>SNAMTNQDRPMKSMSESKCYKNRQVFPQDTNHHHTMFGGTLMANIDEIAAITAMKHAGAQVVAASTDSVDFLKPIKTGDILQYVAMVSYAGTSSMEVVVQIRIDDVFNNKHDLAALSYLTFVALDDEGKPKHVPGVYPEDDVEKWFYDTAPQRVERRKARRIESKQ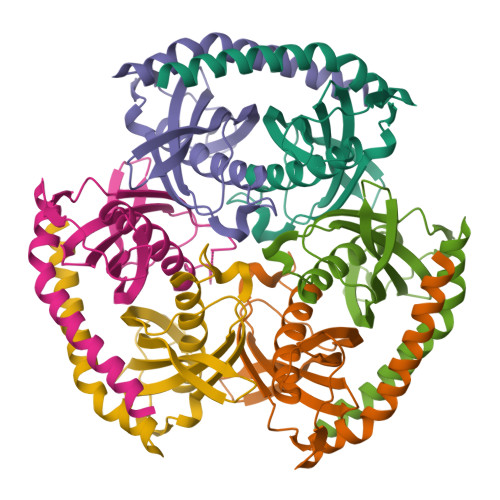TIEYLAQAQHIRD[6x]>GPLGSDQTWVQCDACLKWRKLPDGMDQLPEKWYCSNNPDPQFRNCEVPEEPED[2x];>[2x]A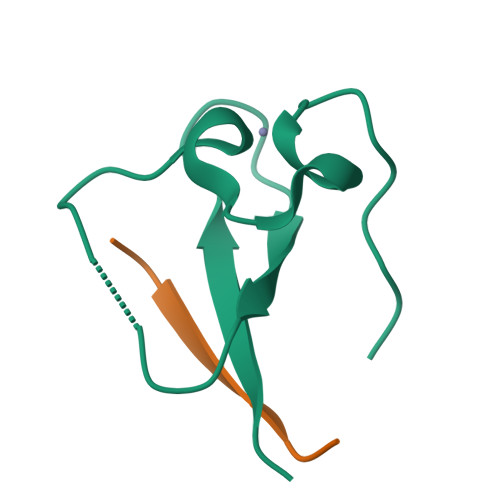RTKQTAR> MVSTQNEPHRFPPDFQWGVATSSYQIEG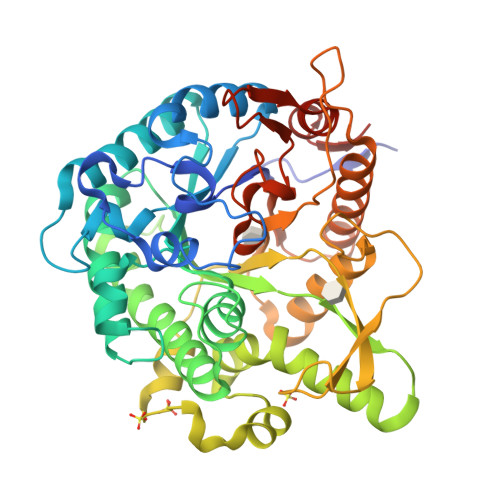AVEADGRSPSIWDTFCARPGAIADGSTGAIANDHYHRYREDIAIMKQLGVNAYRFSIAWPRILPDGRGRVNQAGVDFYERLVDSLLEQGIEPYATLYHWDMPQVQHDRTPWYDRGVVDAFVEYTDVITRRLSDRVKYWMTLNEPWVISFLGYGAGEHAPGLRDKELYLRAAHHVLLAHGKAMPVIRANGNAQTKAGIVLNLNWVNAASDSPEDQAAARRYDQFFNRWFAEPLYNGRYPEELLEWYGRDLVPVQPGDFDIITTPTDFLAVNYYARTTVKAGSTDPMLQVDFVRPPGEYTAMDWEVYPQGLYNILNWLHTDYAPPALYVTANGAAYDDQVSAAGEVDDPQRLAYLEGHFEAAYRAIQAGIPLKGYFVWSLMDNFEWGRGFEKRFGIVFVDYATQQRIIKRSGKWFSQVTRANGLPAPQTTLP>GHMNDLIDTTEMYLRTIYDLEEEGVVPLRARIAERLEQSGGTVSQTVARMERDGLLTVAEDRHLELTKAGRARAISVMRKHRLAERLLVDVIGLEWEQVHLEACRWEHVMSEAVERKLVKLLGNPTTSPYGNPIPGLDELGVGDSVEPVDTDLRRVDEVARSGGGRALVCRIAEHVQLDPDLMSELKKVGVVPGNEIDIVAVAGVNKPIQVQGSEGGTQLQPGIAHAVMV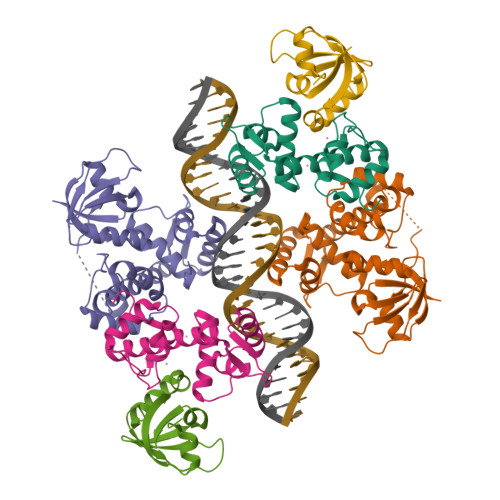RVK[6x]>[5x]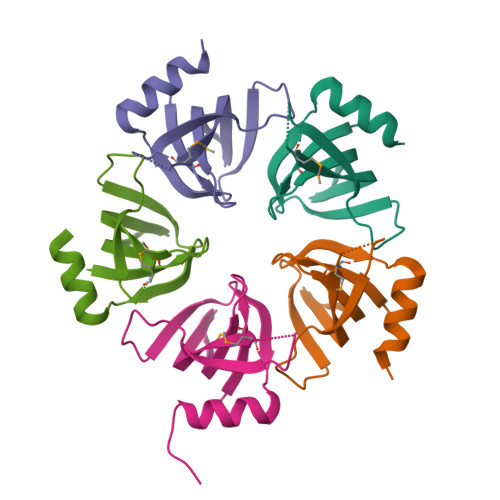GMKNIKIMRLVTGEDIIGNISESQGLITIKKAFVIIPMQATPGKPVQLVLSPWQPYTDDKEIVIDDSKVITITSPKDDIIKSYESHTSEIITPSGLITET> DYKLFITEGYEVGRVNGLAVIGESAGIVLPIIAEVTPSMSKSEGRVIATGRLQEIAREAVMNVSAIIKKYTGRDISNMDVHIQFVGTYEGVEGDSASISIATAVISAIEGIPVDQSVAMTGSLSVKGEVLPVGGVTQKIEAAIQAGLKKVIIPKDNIDDVLLDAEHEGK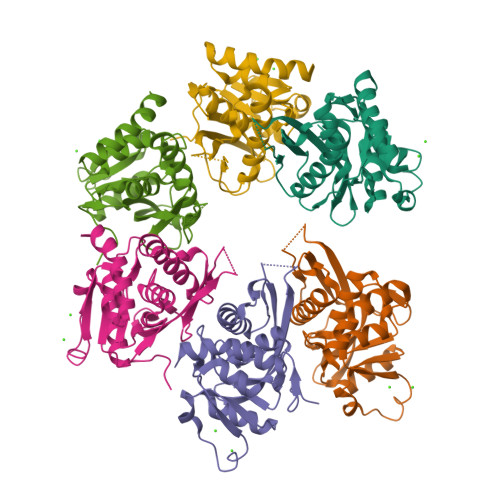IEVIPVSRINEVLEHVLEDGKKKNRLMSKFKELELAAV Engineered small non-antibody protein scaffolds are a promising alternative to antibodies and are especially attractive for use in protein therapeutics and diagnostics. We proved the applicability of this systematic procedure by selecting a monomeric single-domain human protein with a fold different from previously known scaffolds. The newly developed scaffold, called ProBi (Protein Binder), contains two independently mutable surface patches. We demonstrated its functionality by training it as a binder against human interleukin-10, a medically important cytokine.

To generate ProBi-based binders to IL-10, we created a DNA library by randomization of 10 amino acids on one of the ProBi surface patches and used the ribosome display technique to screen for ProBi variants with the highest affinity. The random mutagenesis of these 10 positions gave rise to the maximal diversity of more than 1012 variants, which agreed with the potential diversity suitable for ribosome display. After the fourth selection round of ribosome display, we selected eight random colonies for two-step purification and crystallization trials. We used commercial screens for preliminary crystallization trials and then manually optimized the conditions to get better diffracting crystals. We started the crystallization with seven variants (G14, G21, H25, H33, J61, J70, and J93). We observed a crystallization process of six variants, and only the G21 did not result in any crystal form in our tested screens. Four variants created crystals with low diffraction quality (ranging 6 to 8 Å). Crystallization of the J61 variant resulted in crystals diffracting up to a high resolution (1.2 Å). The fold remains stable even after nine mutations at the selected positions. Because the affinity of the J61 variant to IL-10 was only in the micromolar range we continued in the effort to develop higher affinity binders.

> MAHHHHHHSAALEVLFQGPGQPGFCIKTNSSEGKVFINICHSPSIPPPADVTEEELLQMLEEDQAGFRIPMSLGEPHAELDAKGQGCTAYDVAVNSDFYRRMQNSDFLRLLVIRIARQGLEYKYDLRLAPPWDMMKNRPFMGSISQQNIR>SNAMKKFFIIGTDTEVGKTYISTKLIEVCEHQNIKSLCLKPVASGQSQFSELCEDVESILNAYKHKFTAAEINLISFNQAVAPHIIAAKTKVDISIENLKQFIEDKYNQDLDILFIEGAGGLLTPYSDHT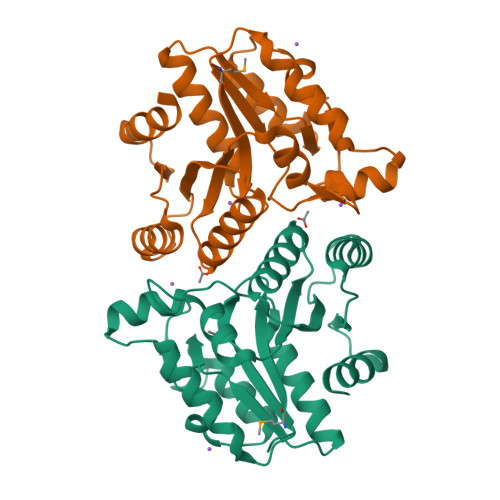TQLDLIKALQIPVLLVSAIKVGCINHTLLTINELNRHNIKLAGWIANCNDSNIKYIDEQINTIEELSGYKCSAKISRNADYLDFIDLSKILISPEENE[2x]> MKKKQIEFEN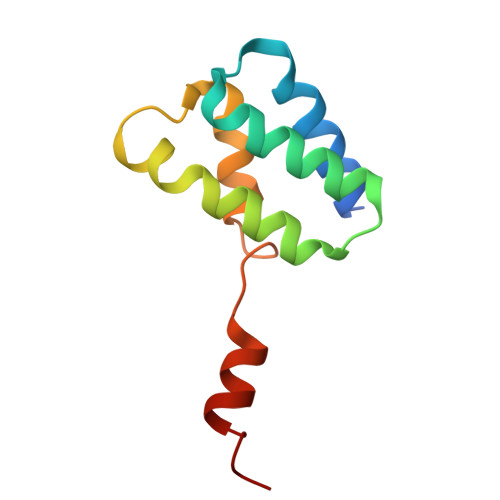ELRSMLATALEKDISQEERNALNIAEKALDNSEYLPKIILNLRKALTPLAINRTLNHDLSELYKFITSSKASNKNLGGGLIMSWGRLF>MMPIKSIVTLDQLEDSEYLFRIVSTVLPHLCLDYKVCDQLKTTFVHPFDILLNNSLGSVTKQDELQAAISKLGINYLIDTTSRELKLFNVTLNAGNIDIINTPINISSETNPIINTHSFYDLPPFTQHLLNIRLTDTEYRARFIGGYIKPDGSDSMDVLAEKKYPDLNFDNTYLFNILYKDVINAPIKEFKAKIVNGVLSRQDFDNLIGVRQYITIQDRPRFD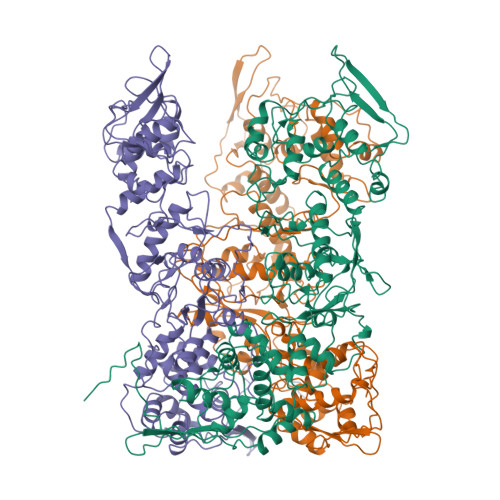DAYNIADAARHYGVNLNTLPLPNVDLTTMPTYKHLIMFEQYFIYTYDRVDIYYNGNKMLFDDEIINFTISMRYQSLIPRLVDFFPDIPVNNNIVLHTRDPQNAAVNVTVALPNVQFVDINRNNKFFINFFNLLAKEQRSTAIKVTKSMFWDGMDYEEYKSKNLQDMMFINSTCYVFGLYNHNNTTYCSILSDIISAEKTPIRVCLLPRVVGGKTVTNLISETLKSISSMTIREFPRKDKSIMHIGLSETGFMRFFQLLRLMADKPHETAIKEVVMAYVGIKLGDKGSPYYIRKESYQDFIYLLFASMGFKVTTRRSIMGSNNISIISIRPRVTKQYIVATLMKTSCSKNEAEKLITSAFDLLNFMVSVSDFRDYQSYRQYRNYCPRYFYAG[3x]> MVDLRTQVLDVPVQETITKDNVPVRVNAVVYFRVVDPVKAVTQVKNYIMATSQISQTTLRSVIGQAHLDELLSERDKLNMQLQRIIDEATDPWGIKVTAVEIKDVELPA

Stomatin is an integral membrane protein that was first identified in human erythrocytes, and is ubiquitously expressed in all tissues. Stomatin is a member of stomatin, prohibitin, flotillin, and HflK/C (SPFH) domain proteins, which are found in the lipid rafts of various cellular membranes. SPFH proteins could function as membrane-bound oligomeric scaffolding proteins in lipid rafts. Mouse stomatin forms a banana-shaped dimer, and Ph stomatin forms a trimer as a building block.

On the other hand, the estimated molecular mass of PhStom (63–234) was 44 kDa, indicating that it forms a dimer based on the molecular mass of its monomer, 20 kDa. The crystal structure of PhStom (63–234) contains residues 64–169, and it forms a banana-shaped dimer in the crystal packing. The structure of PhStom (63–234) contains one molecule in an asymmetric unit. The final model contains residues 64–169, one Na+, and 21 water molecules. Therefore, it is considered that the coiled-coil region of residues 170–234 was degraded during crystallization. The structure of PhStom (63–234) consists of an SPFH domain (residues 64–169) and is nearly the same as that of the SPFH domain of PhStom (56–234). Neighboring symmetry-related molecules with the largest interface area are shown in descending order as sym1 (N-terminal head to N-terminal head interaction), sym2 (C-terminal tail to C-terminal tail interaction), and sym3 (side to side interaction), with areas of 494, 418, and 335 Å2, respectively. Conserved residues such as Leu133, Lys164, and Val166 are located in the interface of sym2. This C-terminal tail to C-terminal tail interaction causes the formation of the banana-shaped dimer as reported in mouse stomatin.> GSHMTTPSRRRLMRDFKKLQEDPPAGVSGAPTEDNILTWEAIIFGPQETPFEDGTFKLSLEFTEEYPNKPPTVKFIS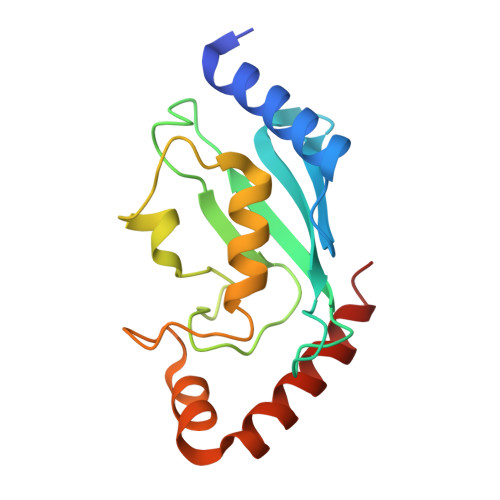KMFHPNVYADGSICLDILQNRWSPTYDVAAILTSIQSLLDEPNPNSPANSLAAQLYQENRREYEKRVQQIVEQSWLNFGE> SSPPVVDTVHGKVLGKFVSLEGFAQPVAIFLGIPFAKPPLGPLRFTPPQPAEPWSFVKNATSYPPMCTQDPKAGQLLSELFTNRKENIPLKLSEDCLYLNIYTPADLTKKNRLPVMVWIHGGGLMVGAASTYDGLALAAHENVVVVTIQYRLGIWGFFSTGDEHSRGNWGHLDQVAALRWVQDNIASFGGNPGSVTIFGEAAGGESVSVLVLSPLAKNLFHRAISESGVALTSVLVKKGDVKPLAEQIAITAGCKTTTSAVMVHCLRQKTEEELLETTLKMKFLSLDLQGDPRESQPLLGTVIDGMLLLKTPEELQAERNFHTVPYMVGINKQEFGWLIPMLMSYPLSEGQLDQKTAMSLLWKSYPLVCIAKELIPEATEKYLGGTDDTVKKKDLFLDLIADVMFGVPSVIVARNHRDAGAPTYMYEFQYRPSFSSDMKPKTVIGDHGDELFSVFGAPFLKEGASEEEIRLSKMVM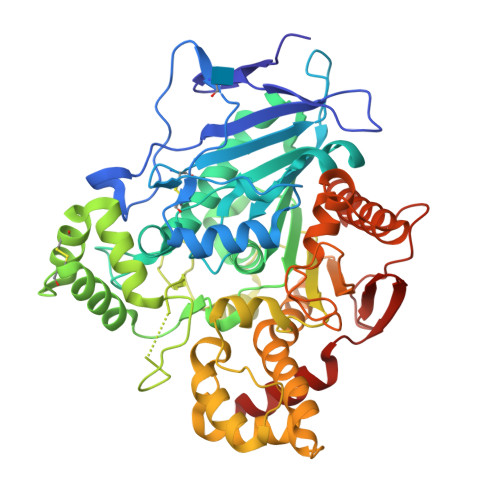KFWANFARNGNPNGEGLPHWPEYNQKEGYLQIGANTQAAQKLKDKEVAFWTNLFAK3’,5’-cyclic uridine monophosphate (cUMP) and 3’,5’-cyclic cytidine monophosphate (cCMP) have been established as bacterial second messengers in the phage defense system, named pyrimidine cyclase system for anti-phage resistance (Pycsar). Until 2021, scientists reported that a group of bacterial nucleotide cyclases, which utilize UTP, and CTP to synthesize cUMP and cCMP, defend against bacteriophage infection, proving that cUMP, and cCMP are authentic second messengers controlling anti-phage defense in prokaryotes. This anti-phage system, termed pyrimidine cyclase system for antiphage resistance (Pycsar), contains a pyrimidine cyclase PycC and a receptor protein with either transmembrane domain (PycTM) or Toll/interleukin-1 receptor domain (PycTIR). Upon phage infections, produced cyclic mono-pyrimidines activates their receptors PycTM, which disrupts membrane integrity by forming transmembrane-spanning pore, or PycTIR, which deplete NAD+, leading to growth arrests and cell deaths, thus protecting the uninfected bacterial populations, a strategy called “abortive infection”. In this study, we aimed to structurally, and functionally characterize both cUMP- and cCMP-synthesizing PycC and cUMP receptor PycTIR.

Among the discovered pyrimidine cyclases, only clade E PycC cyclase can synthesize cCMP products. The native crystals of EaPycC that belongs to space group of I23 were subsequently obtained, which contains two EaPycC molecules in the asymmetric unit. The structure of EaPycC was solved by molecular replacement and refined to 2.2-Å resolution. Each EaPycC molecule has a central seven-stranded β-sheet wrapped around three main α-helices. EaPycC assembles into a head-to-tail homodimer with two symmetric active sites at the dimer interface. However, unlike BcPycC, the N-terminal α helix (α1) of EaPycC packs against α4 and α5 helices in the same protomer instead of extending into the opposing protomer. Another distinct feature found in EaPycC is a C-terminal Y-shaped structure that comprises two anti-parallel β-sheets (β10–β13) near the active sites. The active site of EaPycC contains two conserved catalytic residues D102 and D146 responsible for divalent metal coordination, which superimposed well with those in PaPycC and BcPycC. In contrast to the UTP-recognition residues, Y50, D94, and R97, identified in BcPycC, EaPycC contains strikingly different specificity-determining residues, F100, R142, and Q144, for CTP binding. Indeed, mutating F100, R142, and Q144 to alanine residues abolished the cytidylate cyclase activity of EaPycC, yielding no cCMP products (LC-MS dataset).

>[2x]GMEQKLYKNYADDIAHYLKQGKKNNLQKGLSYEHFSKNLSSHPKMQWVDKTKNEANFRSLSALNTITGQITKYEEKLGAHPSFSHLKNTNDSEYHYIVSMFVDVRNSTGLFKKFDPDVVANICRTIQLATIHTCWYFDGYVHRLQGDGLMVYFGGKGTTKQKAVDNALMAASFISYFVKNDLKNLFEEQGVSRIYTRIGLDFGDDEDTLWHNAGIGECSEVTTTSLHTSLACKMQAQAESNGVVVGDNILPYKSSDKNYFTYKKYKKNGSELPYVYEIPEEYFRYKQHDFNWEKFLKNHPQIQEDEDGNLTFINPSLPPNPRVQQNINHLQQNVSGYKPYLR3-[(1-carboxyethenyl)oxy]-2-hydroxybenzoic acid | C10 H8 O6 | 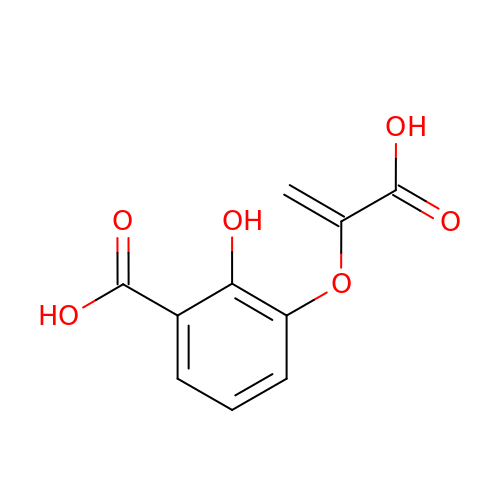RFJWXQPFGYFIBS-UHFFFAOYSA-N>MGNKNTPLNSGKHPDLKIEVAIIGAGTSGLYTAYRLVTDKKFKAHDVQIFDMNNKLGGRLESVIMPGMNFWGELGGMRYLTSQQIVTTLIEGYPLSEKDPNKRTPVLKDKMTPVPFPMGDPSKLLMYLRKERFKQNAWNEAQKKGEKLPTRYYLNENDLGFSSDQLFNKIIYDVLMADPWVAETYGSKIIKGSSVYDYSFKLTSRDWDDIKPKLVYNFPNSPYDQRKVNDIGFWNLIKDQVSQEGYEFLANAGGYYSNTINWNSAEAFPYMVGDFSAGTIYKTIEEGYDSIAYAVANSYMEHEGACIWSENKLLTFTKDHPLTNTHKYELTFLNLKTNTQWKVYANSIVLAMPRKSLELLDQNNFFFNINKNSVLNNNIRSVIMEPAFAILMGFEYPWWKELGIDSGHSITDLPMRQCYYFGTDPETNNSMLLGSYGDMETETFWKALSDDKVLFEVKAAKSASLRELHQLDDVQATKLMVGELMNQLRELHGDTVTIPEPYVTYFKDWTDEPFGAGYHAWKAGFSVENVMPYMRKPLTDEQIHICGEAYSDQQGWVEGAFCEAEKMLQEYFGLDRPYWLSPDYYLGWEHHHHHH[2x]

Progenitor sequence of the assigned 28 sequences was generated by ancestral sequence reconstruction, and the generated sequence exhibited L-lysine oxidase activity; thus, we named the enzyme AncLLysO. AncLLysO has a fold typical of the flavin-dependent amine oxidase (FAO) superfamily —the Rossmann-core fold, which recognizes FAD, and a hot-dog-like fold, which is important for the recognition of substrates. Taken together, we assigned a novel FAD-dependent enzyme, called LLysO and bearing a main L-Lys α-oxidase and promiscuous monooxygenase activity, from the database. The main-chain amino group of L-Lys is deprotonated by an activated solvent water molecule, and the hydride on the main-chain carbon atom is transferred to FAD.

Previous research indicates that, in many FAD-dependent oxidases, the Lys residue at the site would recognize the O2 molecule, which oxidizes the FADH2, and their variants quietly reduce the activity. In AncLLysO, K387 corresponds with the residue, and the activity of the AncLLysO(K387A) variant was reduced below the detection limit of the activity assay as expected. Crystal structures of the L-Lys- and L-Arg-binding forms of AncLLysO(K387A) were determined at 2.4- and 2.2-Å resolution, respectively, using the cocrystallization method. Rearrangement of the active site structure would be induced by the binding of L-Lys. Specifically, the side-chain Y254 moved away from the active site, associating with the cis–trans transformation of G251, and simultaneously the side chains E383 and Y516 flipped into the active site to recognize L-Lys. Next, we attempted to represent structural changes of AncLLysO that are induced by the binding of substrates. Structural comparison between AncLLysO(LF)- (green) and the L-Lys-binding form of AncLLysO(K387A; magenta) are shown in Figure 5D, suggesting that dynamic structural changes could be confirmed at the following residues: 251 to 254, 383, and 516. The active site residues E383 and Y516 moved to the optimal position to recognize the L-Lys associating with the conformational change of the plug loop in AncLLysO. Structural comparison between AncLLysO and other LAAOs may be helpful to predict how AncLLysO exhibits high substrate specificity toward L-Lys. Superimposed structures of AncLLysO(K387A), AncLAAO, and VioA are represented in Figure 5D, indicating that the size of the active site of AncLLysO is narrower than those of AncLAAO and VioA, as the site was formed mainly by bulky aromatic residues (Phe and Tyr). The narrowing of the active site in AncLLysO made binding to amino acids other than L-Lys difficult; therefore, this could be one of the reasons that AncLLysO exhibits high specificity toward L-Lys.>[2x]GSDDSYARVRAVVMTRDDSSGGWLQLGGGGLSSVTVSKTLQPGDSGGTEFLVH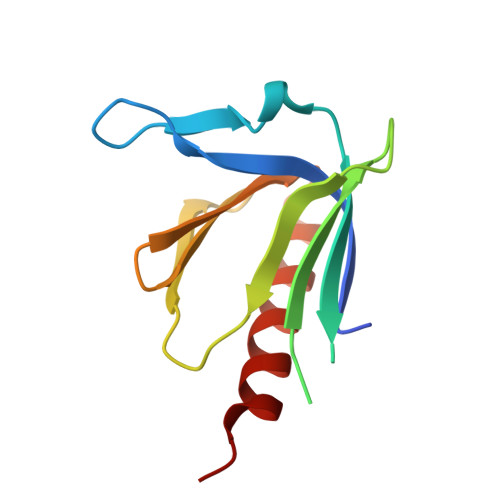GERLRDKTVVLECVLRRDLVYNKVTPTFHHWRIGDKKFGLTFQSPADARAFDRGIRRAIEDLSQG> SWQSYVDDHLMCD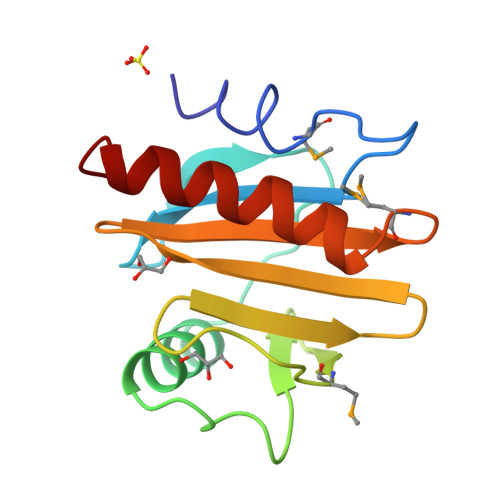VEGNHLTAAAILGQDGSVWAQSAKFPQLKPQEIDGIKKDFEEPGFLAPTGLFLGGEKYMVIQGEQGAVIRGKKGPGGVTIKKTNQALVFGFYDEPMTGGQCNLVVERLGDYLIESEL> MAQAFVDATWPQAAKAAQSLGVPAHFL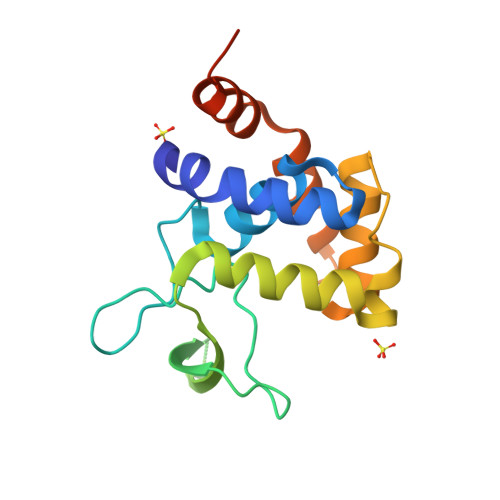VAQAALATGWGKSQIRNKDGTPSYNLFNIKAGSNWTGKVVEARTVEYENGQRKVRVERFRAYDSYEQAFQDYADLVGNSPRYAKVAGKTDGHAFARALQEGGYATDPSYADKLARVINGNALRQRLMASAASARGLEHHHHHH>[4x]MIRSVVIVGGGTAGWMTASYLKAAFDDRIDVTLVESGNVRRIGVGQATFSTVRHFFDYLGLDEREWLPRCAGGYKLGIRFENWSEPGEYFYHPFERLRVVDGFNMAEWWLAVGDRRTSFSEACYLTHRLCEAKRAPRMLDGSLFASQVDESLGRSTLAEQRAQFPYAYHFDADEVARYLSEYAIARGVRHVVDDVQHVGQDERGWISGVHTKQHGEISGDLFVDCTGFRGLLINQTLGGRFQSFSDVLPNNRA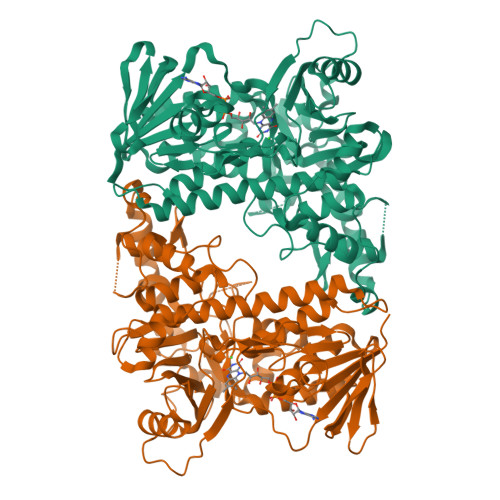VALRVPRENDEDMRPYTTATAMSAGWMWTIPLFKRDGNGYVYSDEFISPEEAERELRSTVAPGRDDLEANHIQMRIGRNERTWINNCVAVGLSAAFVEPLESTGIFFIQHAIEQLVKHFPGERWDPVLISAYNERMAHMVDGVKEFLVLHYKGAQREDTPYWKAAKTRAMPDGLARKLELSASHLLDEQTIYPYYHGFETYSWITMNLGLGIVPERPRPALLHMDPAPALAEFERLRREGDELIAALPSCYEYLASIQ PARP4 is an ADP-ribosyltransferase that resides within the vault ribonucleoprotein organelle. PARP4 is an ADP-ribosyltransferase that uses NAD+ as a substrate to synthesize ADP-ribose modifications on molecules. The PARP1-homology region of PARP4 includes a BRCT fold, a WGR domain, and the catalytic (CAT) domain. However, PARP3 and PARP4 contain the catalytic triad H-Y-E but are considered MARylation enzymes, indicating that other structural features are important determinants of catalytic output.

The PARP4 catalytic domain was crystallized on its own, and in complex with the NAD+-mimic EB47 (32). The CAT/EB47 complex crystals diffracted to 2.95 Å and belong to space group P212121 with two molecules in the asymmetric unit. The refined structure has a crystallographic R/RFREE of 0.215/0.262. While building the model for the HD using the CAT/EB47 diffraction data, it was clear that the HD occupied a significantly different position relative to the ART than that observed with PARP1/2/3. In contrast to PARP1, the PARP4 HD is translated and rotated away from the ART active site, located in a position that does not appear to be an impediment to NAD+ binding. A notable difference between the PARP1 and PARP4 structures is that two helices αA and αB of PARP1 are merged into one continuous helix in PARP4 (referred to as αA/B in PARP4). The presence of the continuous helix αA/B in PARP4 is likely to hold the HD at a specific distance from the ART, essentially maintaining the catalytic region in an open state. The analogous residues in PARP4 (V286 and I289) remain in the interior of the HD fold, suggesting that PARP4 is held in an open and active conformation without requiring the major unfolding event observed in PARP1. The PARP4 catalytic domain crystal structure represents an ‘open’ conformation that is capable of binding substrate NAD+, based on the complex with the NAD+-mimic EB47 and the binding analysis with the non-hydrolyzable NAD+ analog BAD. Our analysis indicates that PARP4 achieves the ‘open’ conformation while maintaining the core fold of the HD.

>[2x]SSEQLQALLLEEVMNSSTLSQEVSDLVEMIWAEALGHLEHMLLKPVNRISLNDVSKAEGILLLVKAALKNGETAEQLQKMMTEFYRLIPHKGTMPKEVNLGLLAKKADLCQLIRDMVNVCETNLSKPNPPSLAKYRALRCKIEHVEQNTEEFLRVRKEVLQNHHSKSPVDVLQIFRVGRVNETTEFLSKLGNVRPLLHGSPVQNIVGILCRGLLLPKVVEDRGVQRTDVGNLGSGIYFSDSLSTSIKYSHPGETDGTRLLLICDVALGKCMDLHEKDFSLTEAPPGYDSVHGVSQTASVTTDFEDDEFVVYKTNQVKMKYIIKFSMPGDQIKD> VHFKDGVYENIPFKVKGRKTPYALSHFG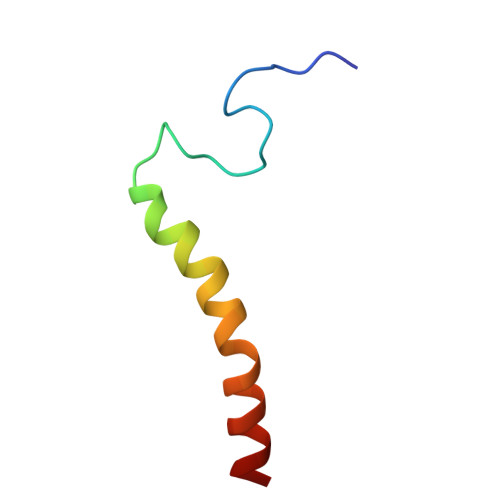FFAIGFAVPFVACYVQLKK> MENKFDHMKLENQLSFLLYASSREMTKQYKPLLDKLNITYPQYLALLLLWEHETLTVKKMGEQLYLDSGTLTPMLKRMEQQGLITRKRSEEDERSVLISLTEDGALL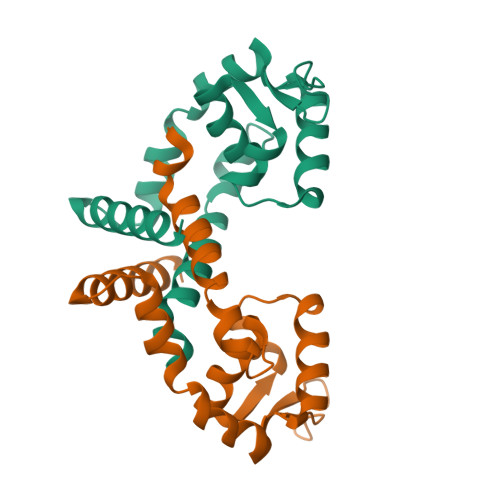KEKAVDIPGTILGLSKQSGEDLKQLKSALYTLLETLHQKN>[4x]TFLHKMGFVVTMLKLIQKKLLDKTCDQVMEFSWSALWNITDETPDNCEMFLNFNGMKLFLDCLKEFPEKQELHRNMLGLLGNVAEVKELRPQLMTSQFISVFSNLLESKADGIEVSYNACGVLSHIMFDGPEAWGVCEPQREEVEERMWAAIQSWDINSRRNINYRSFEPILRLLPQGISPVSQHWATWALYNLVSVYPDKYCPLLIKEGGMPLLRDIIKMATARQETKEMARKVIEHCSNFKEENMDTSR

ZER1 and ZYG11B, the substrate receptors of the Cullin 2-RING E3 ubiquitin ligase (CRL2), recognize N-terminal (Nt) glycine degrons and participate in the Nt-myristoylation quality control through the Gly/N-degron pathway. Here we show that ZER1 and ZYG11B can also recognize small Nt-residues other than glycine. Furthermore, we present the crystal structures of ZER1 and ZYG11B bound to various small Nt-residues and uncover the molecular mechanism of non-acetylated substrate recognition by ZER1 and ZYG11B. In conclusion, we propose that ZER1/ZYG11B not only targets Gly/N-degrons for proteasomal degradation, but it also has the ability to bind a defined selection of non-Ac/N-degrons by a conserved molecular mechanism of substrate recognition and target their degradation through the non-Ac/N-degron pathway.

To understand the molecular basis of ZER1/ZYG11B-mediated binding of non-Gly Nt-residue peptides, we determined the crystal structures of ZER1 bound to either SFLH-, AFLH- or TFLH-peptide, as well as the crystal structures of ZYG11B bound to either SFLH-, AFLH- or CFLH- peptide. In line with our SPOT-array results, ZER1 binds to XFLHVGQD peptides in which X is either Ser (KD of 1.3), Ala (KD of 1.6), Thr (KD of 3.1) or Cys (KD of 3.9) more potently than to the Gly-starting peptide (KD of 4.2). Intriguingly, unlike ZER1, ZYG11B was unable to bind to Nt-Thr, although they adopt similar structural architectures. The free α-amino group of the Nt-residue forms hydrogen bonds with the side chains of Asp556 and Asn597 in ZER1 (the counterparts of Asp 526 and Asn 567 in ZYG11B), respectively. Furthermore, the carbonyl oxygen of the Nt-residue is stabilized by two hydrogen bonds from Asn597 and Trp552 in ZER1 (Asp 567 and Trp522 in ZYG11B). Besides, a strong π-π interaction was formed between the aromatic side chain of F2 and the indole ring of Trp 552 in ZER1 (Trp 522 in ZYG11B), this observation is consistent with our SPOT-array results that ZER1 and ZYG11B prefer an aromatic residue at position 2. Our ITC assays indicated that any alanine mutation of W552, D556, N597 or E600 in ZER1, which would disrupt the direct hydrogen bonds with Nt-residue, abolished the binding to the XFLHVGQD (X = Ser, Ala, Cys or Thr) peptides, highlighting the key role of these hydrogen bonds in mediating Nt-residue recognition. In addition, mutating the third-residue-interacting N553 into alanine caused a significant reduction in substrate binding.> GSMTVEQNVLQQSAAQKHQQTFLNQLREITGINDTQILQQALKDSNGNLELAVAFLTAKNAKTPQQEETTYYQTALPGNDRYISVGSQADTNVIDLTGDDKDDLQRAIALSLAESNRAFRETGITDEEQAISRVLEASIAENKACLKRTPTEVWRDSRNPYDRKRQDKAPVGLKNVGNTCWFSAVIQSLFNLLEFRRLVLNYKPPSNAQDLPRNQKEHRNLPFMRELRYLFALLVGTKRKYVDPSRAVEILKDAFKSNDSQQQDVSEFTHKLLDWLEDAFQMKAEEETDEEKPKNPMVELFYGRFLAVGVLEGKKFENTEMFGQYPLQVNGFKDLHECLEAAMIEGEIESLHSENSGKSGQEHWFTELPPVLTFELSRFEFNQALGRPEKIHNKLEFPQVLYLDRYMHRNREITRIKREEIKRLKDYLTVLQQRLERYLSYGSGPKRFPLVDVLQYALEFASSKPVCTSPVDDIDASSPPSGSIPSQTLPSTTEQQGALSSELPSTSPSSVAAISSRSVIHKPFTQSRIPPDLPMHPAPRHITEEELSVLESCLHRWRTEIENDTRDLQESISRIHRTIELMYSDKSMIQVPYRLHAVLVHEGQANAGHYWAY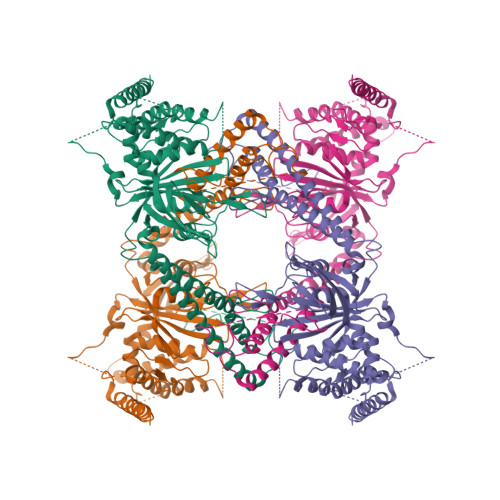IFDHRESRWMKYNDIAVTKSSWEELVRDSFGGYRNASAYCLMYINDKAQFLIQEEFNKETGQPLVGIETLPPDLRDFVEEDNQRFEKELEEWDAQLAQKALQE> GIQGLAKLIADVAPSAIRENDIKSYFGRKVAIDASMSIYQFLIAVRQGGDVLQNEEGETTSHLMGMFYRTIRMMENGIKPVYVFNGKPPQLKSGELAKRSERRAEAEKQLQQAQAAGAEQEVEKFTKRLVKVTKQHNDECKHLLSLMGIPYLDAPSEAEASCAALVKAGKVYAAATEDMDCLTFGSPVLMRHLTASEAKKLPIQEFHLSRILQELGLNQEQFVDLCILLGSDYCESIRGIGPKR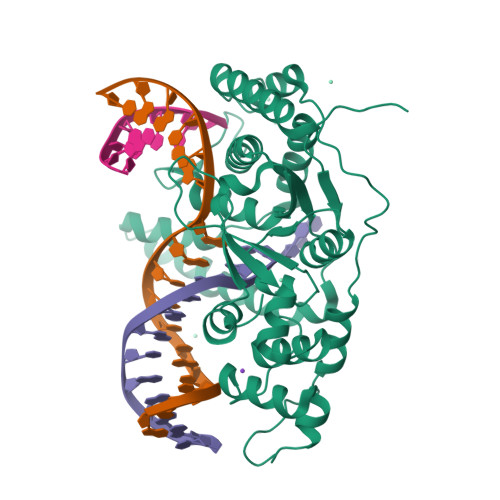AVDLIQKHKSIEEIVRRLDPNKYPVPENWLHKEAHQLFLEPEVLDPESVELKWSEPNEEELIKFMCGEKQFSEERIRSGVKRLSKSRQGSTLEVLFQ(2S)-2-azanyl-6-[(2-bromophenyl)methoxycarbonylamino]hexanoic 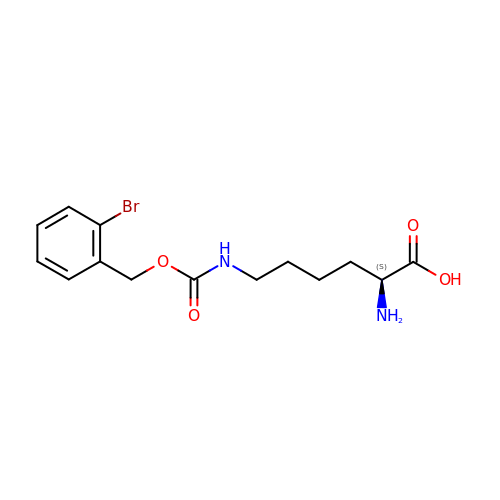acid | C14 H19 Br N2 O4 | YGZWYMNBUCDJRQ-LBPRGKRZSA-N>GSHMNINKQSPIPIYYQIMEQLKTQIKNGELQPDMPLPSEREYAEQFGISRMTVRQA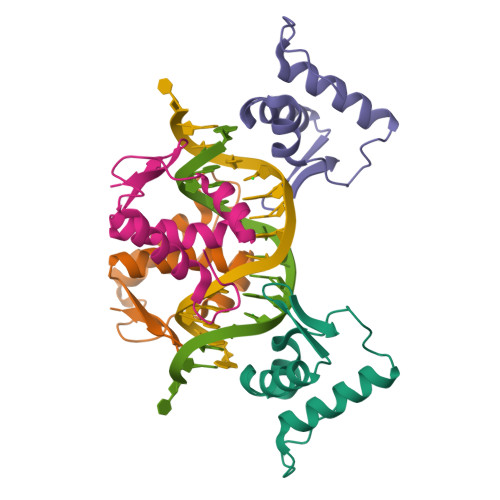LSNLVNEGLLYRLKGRGTFVS[4x]> MNPNQKIITIGSVCMTIGMANLILQIGNIISIWISHSIQLGNQNQIETCNQSVITYENNTWVNQTYVNISNTNFAAGQSVVSVKLAGNSSLCPVSGWAIYSKDNSIRIGSKGDVFVIREPFISCSPLECRTFFLTQGALLNDKHSNGTIKDRSPYRTLMSCPIGEVPSPYNSRFESVAWSASACHDGINWLTIGISGPDNGAVAVLKYNGIITDTIKSWRNNRLRTQESECACVNGSCFTVMTDGPSDGQASYKIFRIEKGKIVKSVEMNAPNYHYEECSCYPDSSEITCVCRDNWHGSNRPWVSFNQNLEYQIGYICSGIFGDNPRPNDKTGSCGPVSSNGANGVKGFSFKYGNGVWIGRTKSISSRNGFEMIWDPNGWTGTDNDFSIKQDIVGINEWSGYSGSFVQHPELTGLDCIRPCFWVELIRGRPKENTIWTSGSSISFCGVNSDTVGWSWPDGAELPFTIDK

Stimulated by the first neuraminidase (NA) crystal structures, the NAIs were designed to interact with the active site of all NA types. We identified a novel isoleucine to arginine change at position 223 (I223R) in the NA of a virus isolated from an immune suppressed child on prolonged oseltamivir and zanamivir therapy. In contrast to the frequently observed H275Y change, which causes selective resistance to oseltamivir, the I223R mutation conferred a resistance phenotype against both oseltamivir and zanamivir. Our results support this suggestion by indicating that a ligand-free form of the pandemic neuraminidase adopts an open conformation. Together with this structure we present the structures of the I223R mutant neuraminidase in complex with oseltamivir and zanamivir to investigate the resistance mechanism of the I223R mutant neuraminidase.

By comparison to the oseltamivir inhibitor constant (KI) of wild type NA, the KI of the I223R mutant increased 48 times and the I223R/H275Y double mutant KI more than 7500 times. The change in the KI for I223R (48-fold) was largely accounted for by an increased dissociation rate constant for the enzyme-inhibitor complex (15-fold) rather than by a reduced association rate constant (kon) (3-fold). In the I223R neuraminidase, this pocket is occupied by the side chain of R223. In displacing the two water molecules seen in the wild-type structure, the arginine makes a hydrogen bond with the side chain of serine 247 (S247). As a result, the side chain of S247 adopts a different rotamer and is oriented towards the active site which enables it to make a second hydrogen bond with glutamic acid 277 (E277). These changes in the structure of the I223R neuraminidase result in shrinkage at the edge of the active site pocket that accommodates the hydrophobic pentoxyl group of oseltamivir. Thus, oseltamivir binding to the active site of I223R neuraminidase requires the reorientation of the S247 and R223 side chains. Moreover, the reorientation of the side-chain of E277, which is required for oseltamivir binding to wild-type neuraminidase, is presumably made even less energetically favorable in the I223R mutant by the need to disrupt the hydrogen bond between S247 and E277. Thus the binding of oseltamivir to the active site of the I223R mutant results not only in changes in the conformation of the side chain of S247 but also in the side-chain of R223 being translated about 1.1 Å out of the active site compared to the mutant ligand-free structure. S247 therefore plays an important role in the decreased sensitivity of the I223R neuraminidase to inhibitors.>INPWFLTGFIDGEGCFRISVTKINRAIDWRVQLFFQINLHEKDRALLESIKDYLKVGKIHISGKNLVQYRIQTFDELTILIKHLKEYPLVSKKRADFELFNTA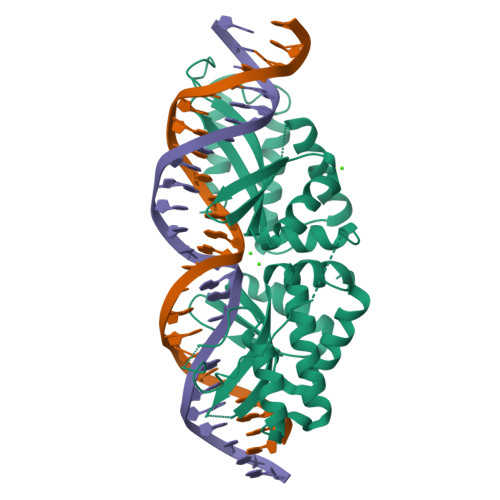HKLIKNNEHLNKEGINKLVSLKASLNLGLSESLKLAFPNVISATRLTDFTVNIPDPHWLSGFASAEGCFMVGIAKSSASSTGYQVYLTFILTQHVRDENLMKCLVDYFNWGRLARKRNVYEYQVSKFSDVEKLLSFFDKYPILGEKAKDLQDFCSVSDLMKSKTHLTEEGVAKIRKIKEGMNRG[2x]>[6x]SNAMGNFHATTIFAVHHNGECAMAGDGQVTMGNAVVMKHTARKVRKLFQGKVLAGFAGSVADAFTLFEMFEGKLEEYNGNLQRAAV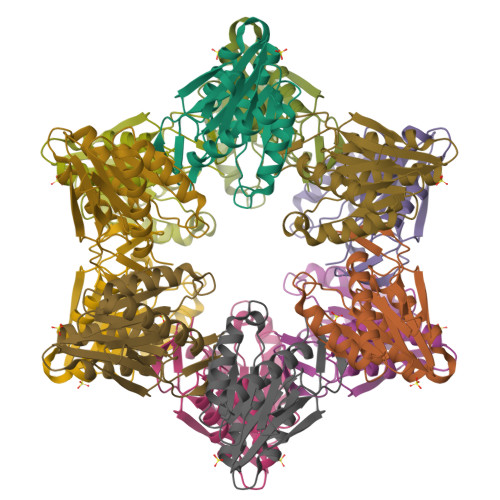EMAKQWRGDKMLRQLEAMLIVMDKTTMLLVSGTGEVIEPDDGILAIGSGGNYALSAGRALKQYASEHLTAKQIAKASLEIAGDICVYTNHNIIVEEL>[2x]HMALFQCDFFSDVLGLSTSMTVILPQETTGQIGMAGGSERREHPTLFLLHGLSDDHTIWLRRTSIERYVAEMGLAVVMPAVHRSFYTDMAHGLQYWTFISEELPALARSFFPLATAREDTFVAGLSMGGYGALKLGMRHPERFAAAASLSGALDITFDPAEHIAMEDDVWVAEQRNIFGDLAALPGSDHDLFALAERMAQSDGPVPKLYQCCGTEDFLYEDNVRFRDHVRGLGLDFMYEESPGEHEWGY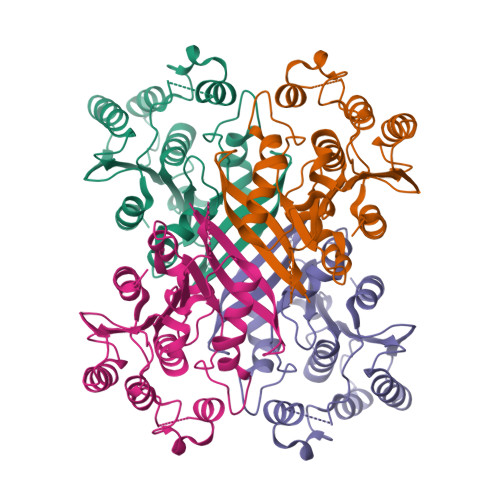WDAQIQRVLAWLPLRPPGTAPA> GSHMMTALETRLSVADGTHAAALRQRLQAALAECRRELAR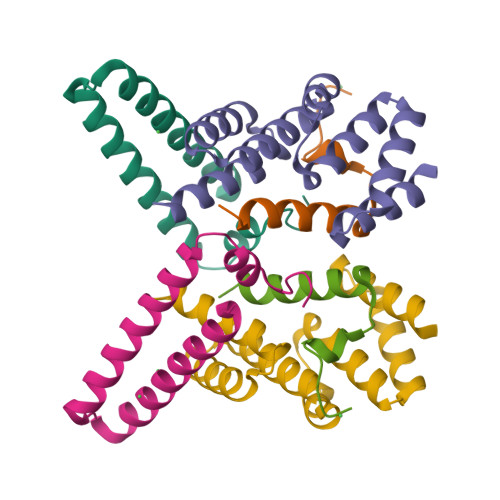GACPERFQFLQQQARALEGGLGILSQLTED;> MHKINKWSVIYNINSTVTRALRDLMQGILQKI;> MDTSLIRELAELALAGSGQHCHEEALCIAEWLERLGQDEAARLIRISSLANQGRYQEALAFAHGNPWPALEPWFALCEWHLGLGAALDRRLAGLGGSSDPALADFAAGMRAQVRT>MAKKTSSKGKLPPGPRPLPLLGNLLQMDRRGLLKSFLRFREKYGDVFTVHLGPRPVVMLCGVEAIREALVDKAEAFSGRGKIAMVDPFFRGYGVIFANGNRWKVLRRFSVTTMRDFGMGKRSVEERIQEEAQCLIEELRKSKGALMDPTFLFQSITANIICSIVFGKRFHYQDQEFLKMLNLFYQTFSLISSVFGQLFELFSGFLKHFPGAHRQVYKNLQEINAYIGHSVEKHRETLDPSAPRDLIDTYLLHMEKEKSNAHSEFSHQNLNLNTLSLFFAGTETTSTTLRYGFLLMLKYPHVAERVYREIEQVIGPHRPPELHDRAKMPYTEAVIYEIQRFSDLLPMGVPHIVTQHTSFRGYIIPKDTEVFLILSTALHDPHYFEKPDAFNPDHFLDANGALKKTEAFIPFSLGKRICLGEGI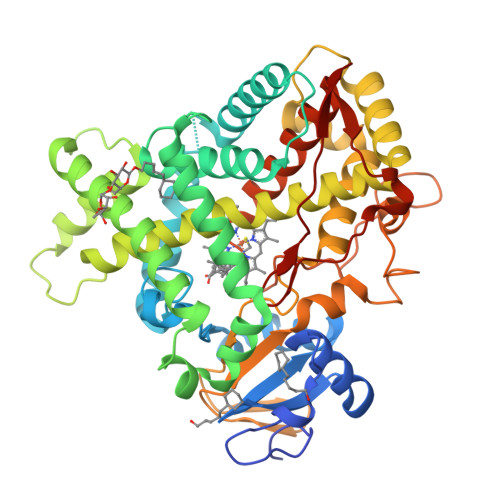ARAELFLFFTTILQNFSMASPVAPEDIDLTPQECGVGKIPPTYQIRFLPRHHHH[2x]>[3x]KPIEIIGAPFSKGQPRGGVEKGPAALRKAGLVEKLKETEYNVRDHGDLAFVDV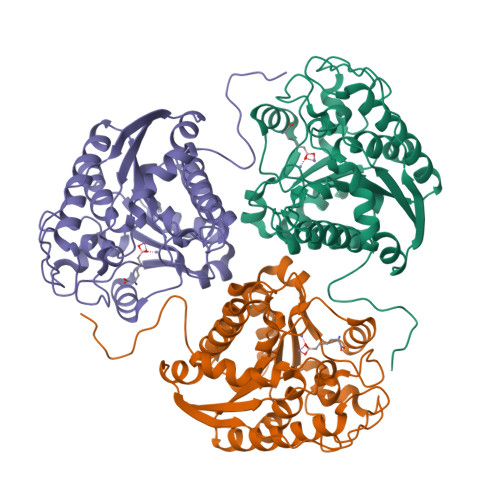PNDSPFQIVKNPRSVGKANEQLAAVVAETQKNGTISVVLGGDHSMAIGSISGHARVHPDLCVIWVDAHTDINTPLTTSSGNLHGQPVAFLLKELKGKFPDVPGFSWVTPCISAKDIVYIGLRDVDPGEHYIIKTLGIKYFSMTEVDKLGIGKVMEETFSYLLGRKKRPIHLSFDVDGLDPVFTPATGTPVVGGLSYREGLYITEEIYKTGLLSGLDIMEVNPTLGKTPEEVTRTVNTAVALTLSCFGTKREGNHKPETDYL>MDSLNFGKALEALKEGKKVSREGWNGKGMFAYYV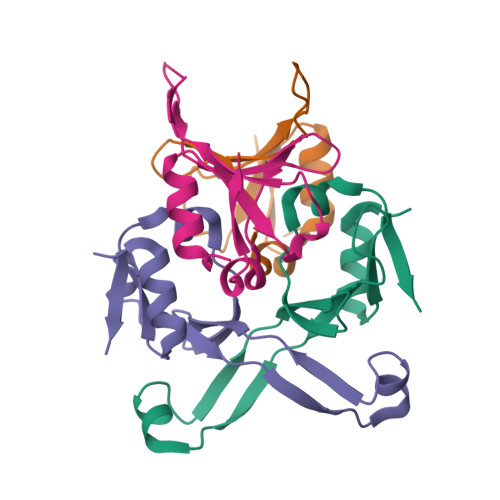PGGVYKSQTDVIKNTFGEEVKYRPYLALKTVDNDIATWTPSVSDILAEDWNIVE[4x]>GUGUCGCAC[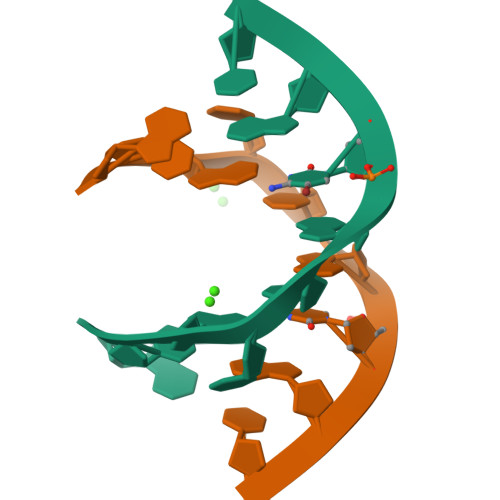4x]>[3x]MSLGGNGREKDHASELRSIFSLKKIADAVNGYEEAKYVVFGIPFDNTSSYRRGSKYAPDSIRGAYVNLESYEYSYGIDLLASGMADLGDMEESEDVEYVIDTVESVVSAVMSDGKIPIMLGGEHSITVGAVRALPKDVDLVIVD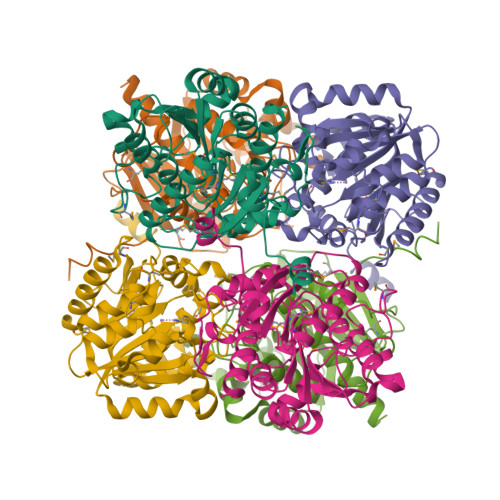AHSDFRSSYMGNKYNHACVTRRALDLLGEGRITSIGIRSVSREEFEDPDFRKVSFISSFDVKKNGIDKYIEEVDRKSRRVYISVDMDGIDPAYAPAVGTPEPFGLADTDVRRLIERLSYKAVGFDIVEFSPLYDNGNTSMLAAKLLQVFIASREKYYKEHIEGHHHHHH>MVVEHPEFLKAGKEPGLQIWRVEKFDLVPVPPNLYGDFFTGDAYVILKTVQLRNGILQYDLHYWLGNECSQDESGAAAIFTVQLDDYLNGRAVQHREVQGFESATFLGYFKSGLKYKKGGVASGFKHVVPNEVVVQRLLQVKGRRVVRATEVPVSWESFNNGDCFILDLGNNIYQWCGSKSNRFERLKATQVSKGIRDNERSGRAQVSVFEEGAEPEAMLQVLGPKPTLPEATEDTVKEDAANRKLAKLYKVSNGAGPMVVSLVADENPFAQGALRSEDCFILDHGKDGKIFVWKGKQANMEERKAALKTASDFISKMDYPKQTQVSVLPEGGETPLFRQFFKNWRDPDQTEGLGLAYLSSHIAHVERVPFDAATLHTSTAMAAQHGMDDDGTGQKQIWRVEGSNKVPVDPATYGQFYGGDSYIILYNYRHGSRQGQIIYNWQGAQSTQDEVAASAILTAQLDEELG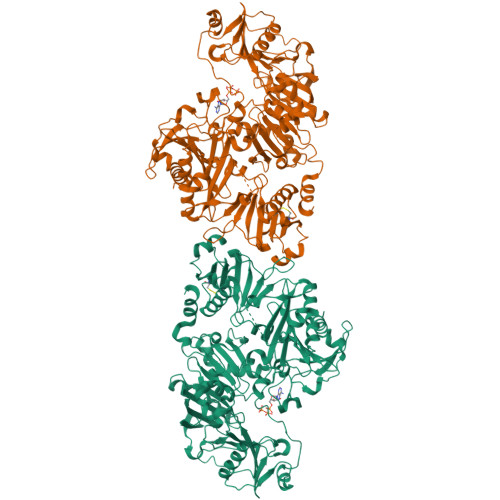GTPVQSRVVQGKEPAHLMSLFGGKPMIVYKGGTSREGGQTAPASTRLFQVRASSSGATRAVEIIPKAGALNSNDAFVLKTPSAAYLWVGAGASEAEKTGAQELLRVLRAQPVQVAEGSEPDSFWEALGGKATYRTSPRLKDKKMDAHPPRLFACSNKIGRFVIEEVPGEFMQEDLATDDVMLLDTWDQVFVWVGKDSQDEEKTEALTSAKRYIDTDPAHRDRRTPITVVKQGFEPPSFVGWFLGWDDSYWSVDPLDRALAELAA[2x]> GSWFFKNLSRKDAERQLLAPGNTHGSFLIRESESTAGSFSLSVRDFDQNQG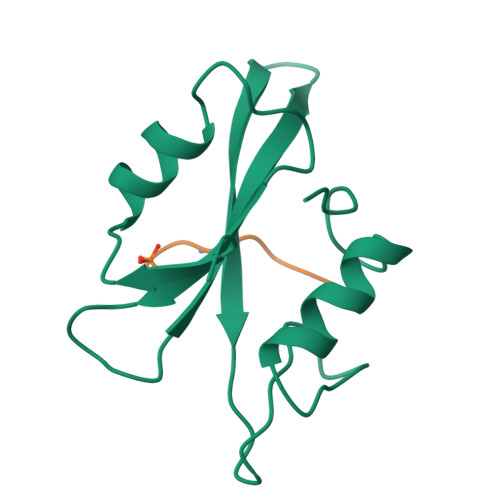EVVKHYKIRNLDNGGFYISPRITFPGLHELVRHYTNASDGLCTRLSR;> PEGDFEEVL(2~{R},3~{S},4~{R},5~{R},6~{S})-2-(hydroxymethyl)-6-(3-naphthalen-2-yl-1~{H}-1,2,4-triazol-5-yl)oxane-3,4,5-triol | C18 H19 N3 O5 | 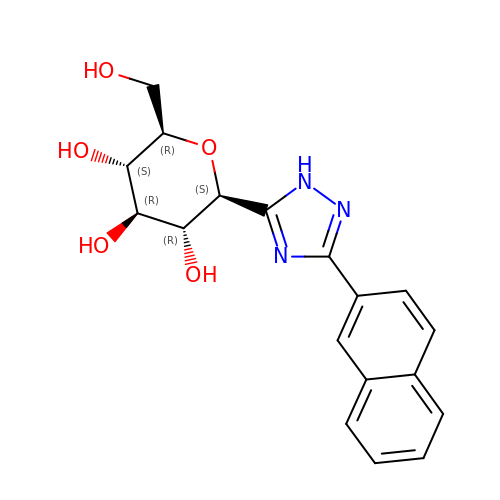FJYFMJBUCUOYNH-IBEHDNSVSA-N> GAMTFTRYSRLRVIAEIRHGDIFHSANIVSSIEFDRDDELFATAGVSRCIKVFDFSSVVNEPADMQCPIVEMSTRSKLSCLSWNKHEKNHIASSDYEGIVTVWDVTTRQSLMEYEEHEKRAWSVDFSRTEPSMLVSGSDDCKVKVWCTRQE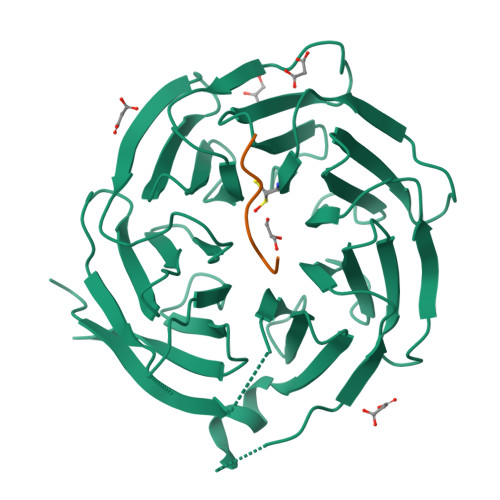ASVINIDMKANICCVKYNPGSSNYIAVGSADHHIHYYDLRNISQPLHVFSGHKKAVSYVKFLSNNELASASTDSTLRLWDVKDNLPVRTFRGHTNEKNFVGLTVNSEYLACGSETNEVYVYHKEITRPVTSHRFGSPDMDDAEEEAGSYFISAVCWKSDSPTMLTANSQGTIKVLVLAA;> XYLQIVPEIHK>MRSMRALSLSLSIFAGAAVATTESTGKASIHDLALQKWTVTNEYGNITVPGKFPSQAHLDLHAAGVIGESNNGLNDFDLRWIAAQNWTYTSKPISGLSKHSDIATWLVFDGLDTYATVKFCDHIVGTPDNQFRQWFYDVSSALASCKSDPVLSINFGSVPRIINAINASDEVQHWPASVVYPFEYPNRQWVRKEQNDFGWDWGPAFSPVGPWQPGRIVQLSKGGELYSLNTDIDIFRKGQFNNFAPDQTAPWVVNASLDFLGTLPKHASMSVIITDASDSRSVLYSGKLEGVTQSDMTVTGSVTIDAHKPKLWWPRDMGNQQLYNITVSVSSAGSKTPILVSQRRVGFRTILFSSGNITDAQIASGITPGNNWHFEINGHEFYAKGANLIPPDAFWPRVTSDRMNRLFDSVESQNFNMLRVWSSGTYLPDWIYDIADERGVLLWSEFQFSDTLYPDSDDFKANVVGEITYNVRRLNHHASLACWMGGNEFENLMLPIAQGADPATYPYVLGQYENLFITTLFNVLAANSHSISYSPCSANNGWLEIDLDLPVPIVERYYNTTSGHIYGDTDFYNYDTSVSFDTSAYPVGRFANEFGFISMPSIQTWQQAVDPEELSFNSTTVILRNHHYPAGGLTRNIHNSTLGQVEMTLAVERYYPTPDKTDPVANFSSWCHATQLFQADMYKSEIQFYRRGSGLPERQLGSLYWQLNDIWQAPTWAGLEYDGRWKV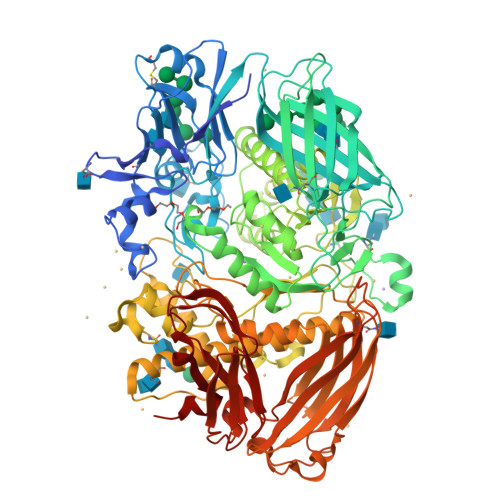LPYVSRRTYEHVIASAFWNYTANELEIWVTSDLWEPVAGEVSLTWVDLKGKPIANNAGMTKSTKFNVGAINTTQIITANIQSDLKIPDTSDAVLVIELTAHGKLPNAASSKTTTFTHHNHFLPVWPNQAKVSDPKLHLSYNKSTKKFTVEATAGVSLYTWLTHPAGVLGFFDDNAFVLRPGEKKEVGFTLQQDTTGGKWTEQVTVESLWDLTTP[2x]> G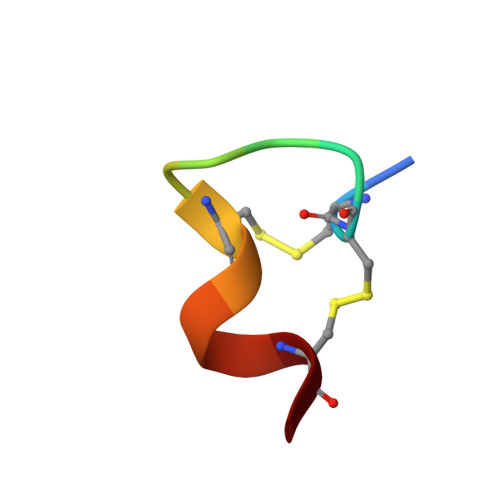CCSDPRCRYRCR>GSMGKPFFTRNPSELKGKFIHTKLRKSSRGFGFTVVGGDEPDEFLQIKSLVLDGPAALDGKMETGDVIVSVNDTCVLGHTHAQVVKIFQSIPIGASVDLELCRGYPLGSSAYGSVKAYTNFDAERDALNIETAIKTKGVDEVTIVNILTNRSNEQRQDIAFAYQRRTKKELASALKSALSGHLETVILGLLKTPAQYDASELKASMKGLGTDEDSLIEIICSRTNQELQEINRVYKEMYKTDLEKDIISDTSGDFRKLMVALAKGRRAEDGSVIDYELIDQDARDLYDAGVKRKGTDVPKWISIMTERSV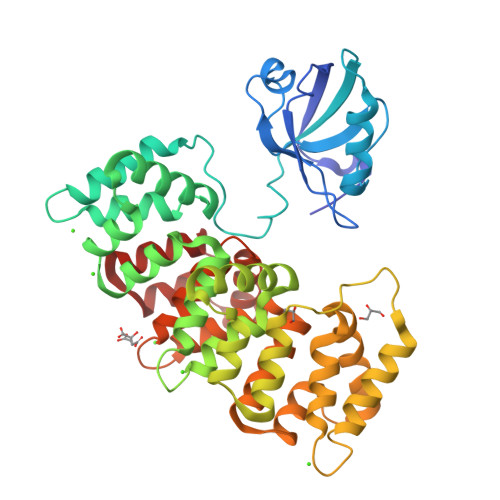PHLQKVFDRYKSYSPYDMLESIRKEVKGDLENAFLNLVQCIQNKPLYFADRLYDSMKGKGTRDKVLIRIMVSRSEVDMLKIRSEFKRKYGKSLYYYIQQDTKGDYQKALLYLCGGDD[2x];> SSRTRREEQL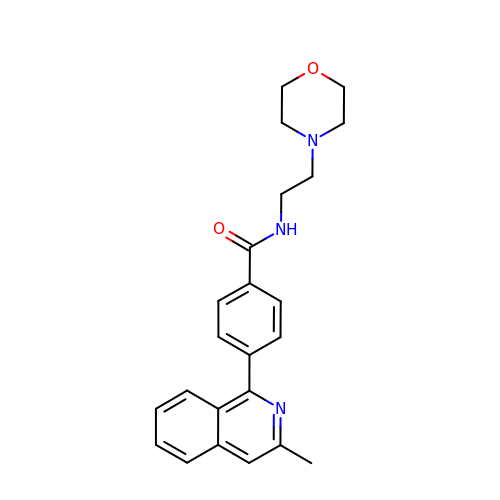4-(3-methylisoquinolin-1-yl)-N-[2-(morpholin-4-yl)ethyl]benzamide | C23 H25 N3 O2 | TUUADNJAZQZKLA-UHFFFAOYSA-N> HPIIQIDRSFMLLILERSTRSILF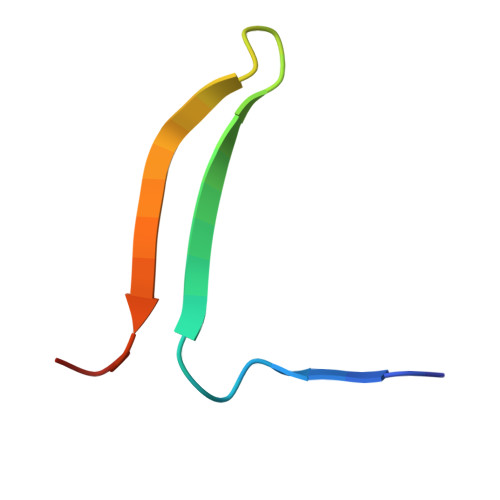LGKVVNPTEA>GSHMGHWSQGLKISMQDPKMQVYKDEQVVVIKDKYPKARYHWLVLPWTSISSLKAVAREHLELLKHMHTVGEKVIVDFAGSSKLRFRLGYHAIPSMSHVHLHVISQDFDSPCLKNKKHWNSFNTEYFLESQAVIEMV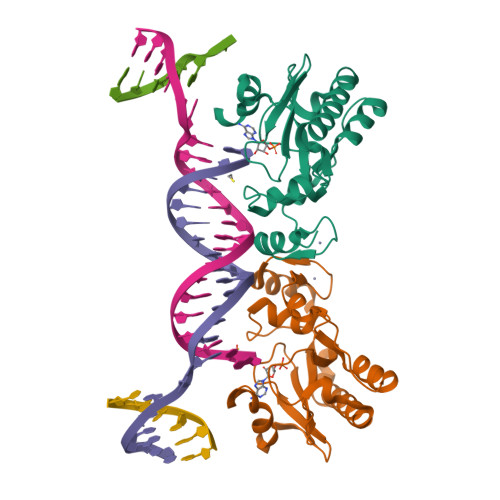QEAGRVTVRDGMPELLKLPLRCHECQQLLPSIPQLKEHLRKHWTQ[2x]> MNLE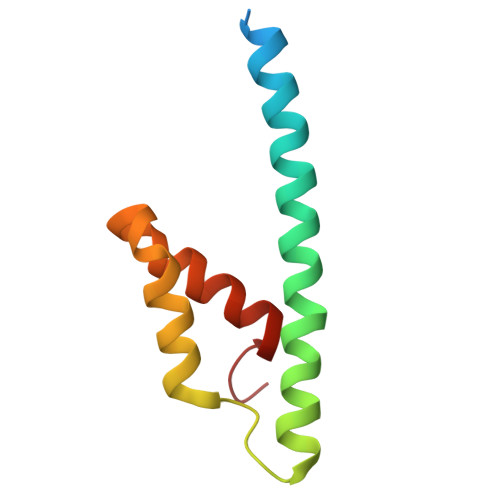MLESQPVPEIDTLREEIDRLDAEILALVKRRAEVSKAIGKARMASGGTRLVHSREMKVIERYSELGPDGKDLAILLLRLGRGRLGH> MKVVNLKQAILQAWKERWSDYQWAINMKKFFPKGATWDILNLADALLEQAMIGPSPNPLILSYLKYAISSQMVSYSSVLTAISKFDDFSRDLCVQALLDIMDMFCDRLSCHGKAEECIGLCRALLSALHWLLRCTAASAERLREGLEAGTPAAGEKQLAMCLQRLEKTLSSTKNRALLHIAKLEEASSWTAIEHSLLKLGEILANLSNPQLRSQAEQCGTLIRSIPTMLSVHAEQMHKTGFPTVHAVILLEGTMNLTGETQSLVEQLTMVKRMQHIPTPLFVLEIWKACFVGLIESPEGTEELKWTAFTFLKIPQVLVKLKKYSHGDKDFTEDVNCAFEFLLKLTPLLDKADQRCNCDCTNFLLQECGKQGLLSEASVNNLMAKRKADREHAPQQKSGENANIQPNIQLILRAEPTVTNILKTMDADHSKSPEGLLGVLGHMLSGKSLDLLLAAAAATGKLKSFARKFINLNEFTTYGSEESTKPASVRALLFDISFLMLCHVAQTYGSEVIL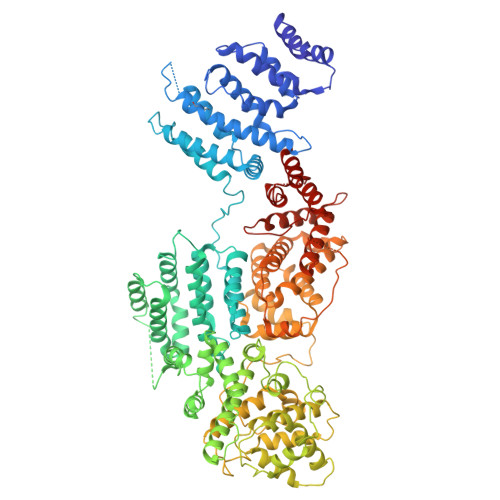SESRTGAEVPFFETWMQTCMPEEGKILNPDHPCFRPDSTKVESLVALLNNSSEMKLVQMKWHEACLSISAAILEILNAWENGVLAFESIQKITDNIKGKVCSLAVCAVAWLVAHVRMLGLDEREKSLQMIRQLAGPLFSENTLQFYNERVVIMNSILERMCADVLQQTATQIKFPSTGVDTMPYWNLLPPKRPIKEVLTDIFAKVLEKGWVDSRSIHIFDTLLHMGGVYWFCNNLIKELLKETRKEHTLRAVELLYSIFCLDMQQVTLVLLGHILPGLLTDSSKWHSLMDPPGTALAKLAVWCALSSYSSHKGQASTRQKKRHREDIEDYISLFPLDDVQPSKLMRLLSSNEDDANILSSPTDRSMSSSLSASQLHTVNMRDPLNRVLANLFLLISSILGSRTAGPHTQFVQWFMEECVDCLEQGGRGSVLQFMPFTTVSELVKVSAMSSPKVVLAITDLSLPLGRQVAAKAIAAL>MGHHHHHHMFSDLRDKVVIVTGASMGIGRAIAERFVDEGSKVIDLSIHDPGEAKYDHIECDVTNPDQVKASIDHIFKEYGSISVLVNNAGIESYGKIESMSMGEWRRIIDVNLFGYYYASKFAIPYMIRSRDPSIVNISSVQASIITKNASA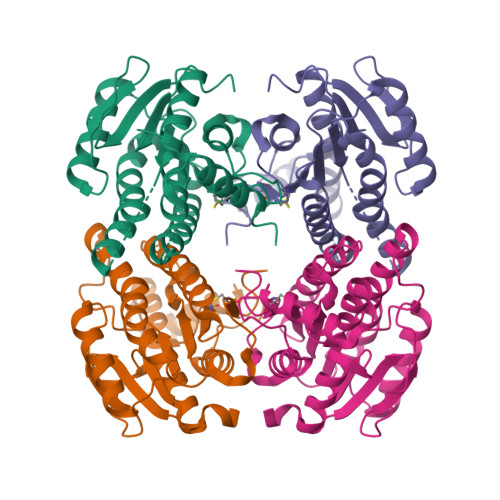YVTSKHAVIGLTKSIALDYAPLLRCNAVCPATIDTPLVRKAAELEVGSDPMRIEKKISEWGHEHPMQRIGKPQEVASAVAFLASREASFITGTCLYVDGGLSIRA[2x]>[2x]APRKFFVGGNWKMNGDKKS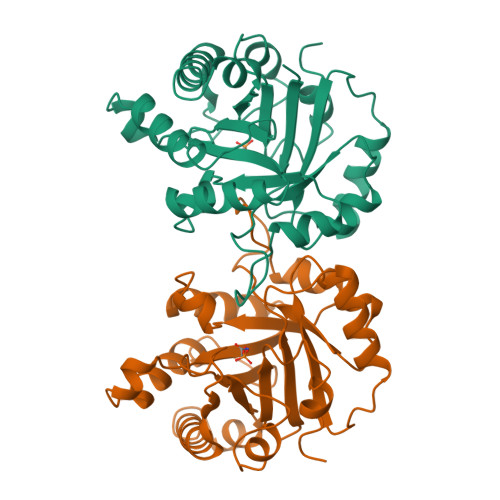LGELIHTLNGAKLSADTEVVCGAPSIYLDFARQKLDAKIGVAAQNCYKVPKGAFTGEISPAMIKDIGAAWVILGHPERRHVFGESDELIGQKVAHALAEGLGVIACIGEKLDEREAGITEKVVFEQTKAIADNVKDWSKVVLAYEPVWAIGTGKTATPQQAQEVHEKLRGWLKTHVSDAVAQSTRIIYGGSVTGGNCKELASQHDVDGFLVGGASLKPEFVDIINAKH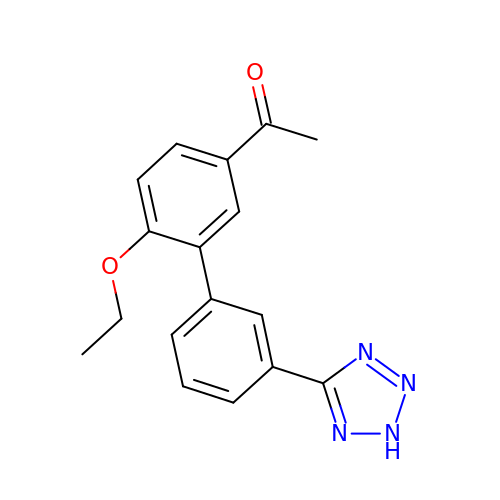1-[4-ethoxy-3-[3-(2~{H}-1,2,3,4-tetrazol-5-yl)phenyl]phenyl]ethanone | C17 H16 N4 O2 | XRDCFDYQIVETFM-UHFFFAOYSA-N> MSRLEIYSPEGLRLDGRRW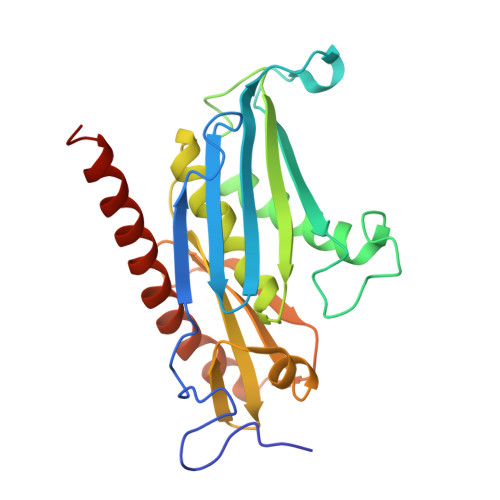NELRRFESSINTHPHAADGSSYMEQGNNKIITLVKGPKEPRLKSQMDTSKALLNVSVNITKFSKFERSKSSHKNERRVLEIQTSLVRMFEKNVMLNIYPRTVIDIEIHVLEQDGGIMGSLINGITLALIDAGISMFDYISGISVGLYDTTPLLDTNSLEENAMSTVTLGVVGKSEKLSLLLVEDKIPLDRLENVLAIGIAGAHRVRDLMDEELRKHAQKRVSNASAR Scribble (Scrib) is a multidomain polarity protein and member of the leucine-rich repeat and PDZ domain (LAP) protein family. The tumor-suppressive activity of Scrib correlates with its membrane localization. Here, we identify the cell adhesion receptor TMIGD1 as a membrane anchor of Scrib. TMIGD1 directly interacts with Scrib through a PDZ domain-mediated interaction and recruits Scrib to the lateral membrane domain in epithelial cells.

We examined the structural basis of this putative binding interface by determining the crystal structure of the isolated Scrib PDZ1 domain in complex with an 8-mer peptide representing the C-terminal region of TMIGD1 which includes the PBM (-DPHSETALCOOH, PBM underlined). The PDZ1:TMIGD1 structure was refined to a resolution of 1.9 Å with a final Rfree of 0.222. The TMIGD1 peptide engaged with the PDZ1 domain via the well-conserved canonical ligand binding groove located between the β2 strand and the α2 helix. Binding of TMIGD1 to Scrib PDZ1 does not alter the overall domain configuration of Scrib PDZ1 as a superimposition of ligand-free Scrib PDZ1 with the Scrib PDZ1:TMIGD1 yielded a root-mean-square deviation of 0.44 Å, with differences between the two structures primarily due to changes in local side chain conformations. Close examination of Scrib PDZ1:TMIGD1 peptide complex revealed several direct interactions that are formed between the peptide and the PDZ1 domain. The C-terminal carboxyl group of the TMIGD1 peptide docks in the conserved hydrophobic pocket of PDZ1, interacting with the main chain L738PDZ1, G739PDZ1 and I740PDZ1. Furthermore, a network of hydrogen bonds is observed between PDZ1 and TMIGD1 including interactions mediated by PDZ domain side chains (H793PDZ1:T260TMIGD1, S748PDZ1:S258TMIGD1, T749PDZ1:D255TMIGD1) and interactions mediated by the PDZ domain main chain (I742PDZ1:A261TMIGD1, I742PDZ1:T260TMIGD1, G744PDZ1:S258TMIGD1, T749PDZ1:P256TMIGD1). Lastly, a salt bridge is found between R762PDZ1 and E259TMIGD1. A comparison of Scrib PDZ1 complexes with known PBM ligands reveals that key interactions are conserved in the Scrib/PDZ1 – TMIGD1 PBM complex. All hydrogen bonds observed in previously characterized Scrib:PBM interactions are recapitulated in the Scrib/PDZ1 – TMIGD1 PBM structure.

> DPHSETAL;> LLIEPARIEEEELTLTILRQTGGLGISIAGGKGSTPYKGDDEGIFISRVSEEGPAARAGVRVGDKLLEVNGVALQGAEHHEAVEALRGAGTAVQMRVWRERM> KFESKAALLAARGPEELLCFTERLEDLVCFWEEAASAGVGPGNYSFSYQLEDEPWKLCRLHQAPTARGAVRFWCSLPTADTSSFVPLELRVTAASGAPRYHRVIHINEVVLLDAPVGLVARLADESGHVVLRWLPPPETPMTSHIRYEVDVSAGNGAGSVQRVEILEGRTECVLSNLRGRTRYTFAVRARMAEPSFGGFW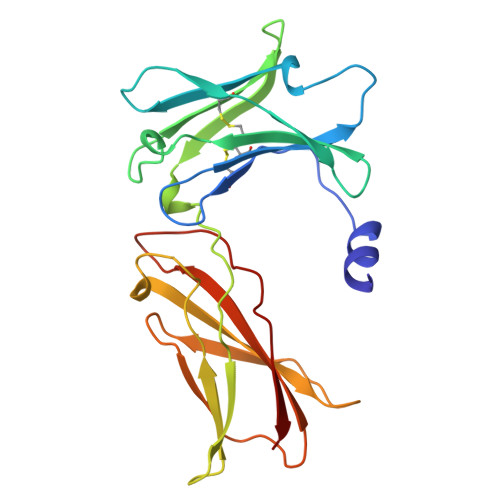SAWSEPVSLLT> MLQCTALVLKSQHKNVLRKGRPHMQKYKELNRWQREAQGITKWEQGHSHRPQPYVERFNPEGAGLTRG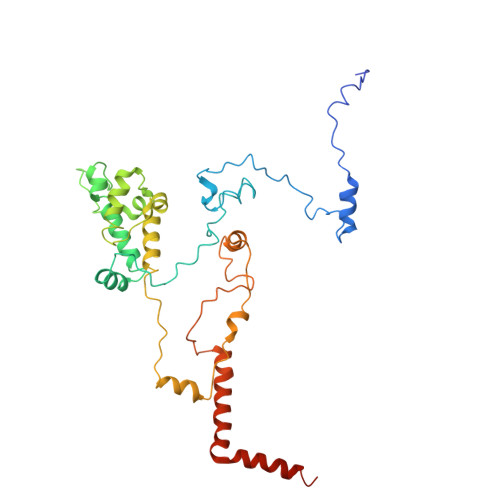TSAYAWKWWHTQYPWLPNVAPADYVPPSPRGIRPAAWDDEFADVVLSMSDEEIQSYLLDKLTEVIFAETQRDGYELRRLDFEGKPLTELPERRIIENFVFEEETLRERVLDRVVEGVFRLVPTSTDRLELKSVANIIDFVLTHVTVARKPLQHEIPEAARTVMRSHPLQPQLGFVHALPTDNRDAVVQEWERMHHLDWQFGKAVYEPRSAENERGNLTWLREVRHHEAREAFQADVDSGEARRRHMAKIKAAAQVPHTGTTSQ> SFK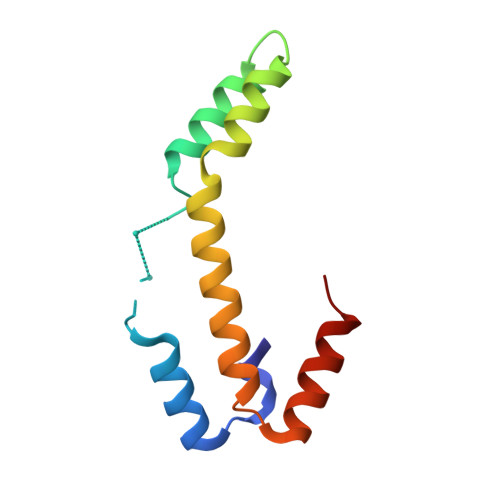DLNLTDAQKQQIREIMKGQRDQMKRPPLEERRAMHDIIASDTFDKVKAEAQIAKMEEQRKANMLAHMETQNKIYNILTPEQKKQFNANFEKRLT> MKIVYWSGTGNTEKMAELIAKGIIESGKDVNTINVSDVNIDE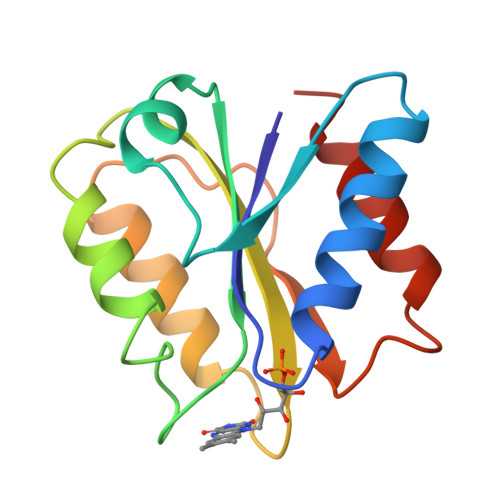LLNEDILILGCSAMGDEVLEESEFEPFIEEISTKISGKKVALFGSYGWGDGKWMRDFEERMNGYGCVVVETPLIVQNEPDEAEQDCIEFGKKIANI> MGFVRQIQLLLWKNWTLRKRQKIRFVVELVWPLSLFLVLIWLRNANPLYSHHECHFPNKAMPSAGMLPWLQGIFCNVNNPCFQSPTPGESPGIVSNYNNSILARVYRDFQELLMNAPESQHLGRIWTELHILSQFMDTLRTHPERIAGRGIRIRDILKDEETLTLFLIKNIGLSDSVVYLLINSQVRPEQFAHGVPDLALKDIACSEALLERFIIFSQRRGAKTVRYALCSLSQGTLQWIEDTLYANVDFFKLFRVLPTLLDSRSQGINLRSWGGILSDMSPRIQEFIHRPSMQDLLWVTRPLMQNGGPETFTKLMGILSDLLCGYPEGGGSRVLSFNWYEDNNYKAFLGIDSTRKDPIYSYDRRTTSFCNALIQSLESNPLTKIAWRAAKPLLMGKILYTPDSPAARRILKNANSTFEELEHVRKLVKAWEEVGPQIWYFFDNSTQMNMIRDTLGNPTVKDFLNRQLGEEGITAEAILNFLYKGPRESQADDMANFDWRDIFNITDRTLRLVNQYLECLVLDKFESYNDETQLTQRALSLLEENMFWAGVVFPDMYPWTSSLPPHVKYKIRMDIDVVEKTNKIKDRYWDSGPRADPVEDFRYIWGGFAYLQDMVEQGITRSQVQAEAPVGIYLQQMPYPCFVDDSFMIILNRCFPIFMVLAWIYSVSMTVKSIVLEKELRLKETLKNQGVSNAVIWCTWFLDSFSIMSMSIFLLTIFIMHGRILHYSDPFILFLFLLAFSTATIMLCFLLSTFFSKASLAAACSGVIYFTLYLPHILCFAWQDRMTAELKKAVSLLSPVAFGFGTEYLVRFEEQGLGLQWSNIGNSPTEGDEFSFLLSMQMMLLDAAVYGLLAWYLDQVFPGDYGTPLPWYFLLQESYWLGGEGCSTREERALEKTEPLTEETEDPEHPEGIHDSFFEREHPGWVPGVCVKNLVKIFEPCGRPAVDRLNITFYENQITAFLGHNGAGKTTTLSILTGLLPPTSGTVLVGGRDIETSLDAVRQSLGMCPQHNILFHHLTVAEHMLFYAQLKGKSQEEAQLEMEAMLEDTGLHHKRNEEAQDLSGGMQRKLSVAIAFVGDAKVVILDQPTSGVDPYSRRSIWDLLLKYRSGRTIIMSTHHMDEADLLGDRIAIIAQGRLYCSGTPLFLKNCFGTGLYLTLVRKMKNIQSQRKGSEGTCSCSSKGFSTTCPAHVDDLTPEQVLDGDVNELMDVVLHHVPEAKLVECIGQELIFLLPNKNFKHRAYASLFRELEETLADLGLSSFGISDTPLEEIFLKVTEDSDSGPLFAGGAQQKRENVNPRHPCLGPREKAGQTPQDSNVCSPGAPAAHPEGQPPPEPECPGPQLNTGTQLVLQHVQALLVKRFQHTIRSHKDFLAQIVLPATFVFLALMLSIVIPPFGEYPALTLHPWIYGQQYTFFSMDEPGSEQFTVLADVLLNKPGFGNRCLKEGWLPEYPCGNSTPWKTPSVSPNITQLFQKQKWTQVNPSPSCRCSTREKLTMLPECPEGAGGLPPPQRTQRSTEILQDLTDRNISDFLVKTYPALIRSSLKSKFWVNEQRYGGISIGGKLPVVPITGEALVGFLSDLGRIMNVSGGPITREASKEIPDFLKHLETEDNIKVWFNNKGWHALVSFLNVAHNAILRASLPKDRSPEEYGITVISQPLNLTKEQLSEITVLTTSVDAVVAICVIFSMSFVPASFVLYLIQERVNKSKHLQFISGVSPTTYWVTNFLWDIMNYSVSAGLVVGIFIGFQKKAYTSPENLPALVALLLLYGWAVIPMMYPASFLFDVPSTAYVALSCANLFIGINSSAITFILELFENNRTLLRFNAVLRKLLIVFPHFCLGRGLIDLALSQAVTDVYARFGEEHSANPFHWDLIGKNLFAMVVEGVVYFLLTLLVQRHFFLSQWIAEPTKEPIVDEDDDVAEERQRIITGGNKTDILRLHELTKIYPGTSSPAVDRLCVGVRPGECFGLLGVNGAGKTTTFKMLTGDTTVTSGDATVAGKSILTNISEVHQNMGYCPQFDAIDELLTGREHLYLYARLRGVPAEEIEKVANWSIKSLGLTVYADCLAGTYSGGNKRKLSTAIALIGCPPLVLLDQPTTGMDPQARRMLWNVIVSIIREGRAVVLTSHSMEECEALCTRLAIMVKGAFRCMGTIQHLKSKFGDGYIVTMKIKSPKDDLLPDLNPVEQFFQGNFPGSVQRERHYNMLQFQVSSSSLARIFQLLLSHKDSLLIEEYSVTQTTLDQVFVNFAKQQTESHDLPLHPRAAGASRQAQD

ABCA4, also known as the Rim protein or ABCR, is an ATP-binding cassette (ABC) transporter essential to vision. Transporter assays have demonstrated that ABCA4 actively transports N-retinylidene-PE across disc membranes. These studies provide direct evidence that ABCA4 is an ATP-driven importer, transporting N-retinylidene-PE from the luminal to the cytoplasmic side of the disc membrane in photoreceptor cells. It consists of two homologous halves, each containing a transmembrane domain (TMD), an exocytoplasmic domain (ECD), a cytoplasmic nucleotide binding domain (NBD), and a regulatory domain (RD). Over 800 mutations in the ABCA4 gene cause Stargardt disease, the most common form of inherited macular degeneration.

The final model contains 2 ATP molecules, 8 lipid molecules, and 1920 residues. In the presence of ATP and absence of substrate, ABCA4 exhibits a conformation very different from that of the ATP-free structure. The two NBDs form a closed dimer. The two TMDs are also in close contact, leaving no cavity at their interface. The ECDs are positioned differently from that of the ATP-free form, placing the hollow channel directly above the EH3-turn-EH4 cleft. In ABCA4, this role is fulfilled by the mainchain carboxyl group of T2070 in ATPase site 1 and the side chain of K1054 and mainchain carboxyl of D1061 in ATPase site 2. For example, in the ATP-bound conformation, D1102 in NBD1 forms a hydrogen bond with H2202 in RD2, and R2107 in NBD2 forms salt bridges with E1270 in PH1. The helical subdomain of NBD1 moves together with TMD1. This twisting motion, not seen in any other ABC transporter, places helices TM1 and TM2 within van der Waals’ contact with TM8 and TM11, closing the TM cavity completely. ATP binding induces a major conformational change that closes the transmembrane pathway to release substrate.>[2x]MGHHHHHHHHEFIPSNTDYPGPHHFEVTFQQSSTAKSATWTYSPLLKKLYCQIAKTCPIQIK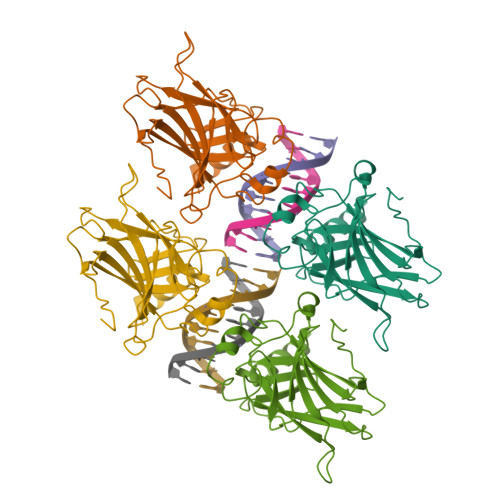VSTPPPPGTAIRAMPVYKKAEHVTDVVKRCPNHELGRDFNEGQSAPASHLIRVEGNNLSQYVDDPVTGRQSVVVPYEPPQVGTEFTTILYNFMCNSSCVGGMNRRPILIIITLEMRDGQVLGRRSFEGRICACPGRDRKADEDHYREQ> MMVEVRFFGPIKEENFFIKANDLKELRAILQEKEGLKEWLGVCAIALNDHLIDNLNTPLKD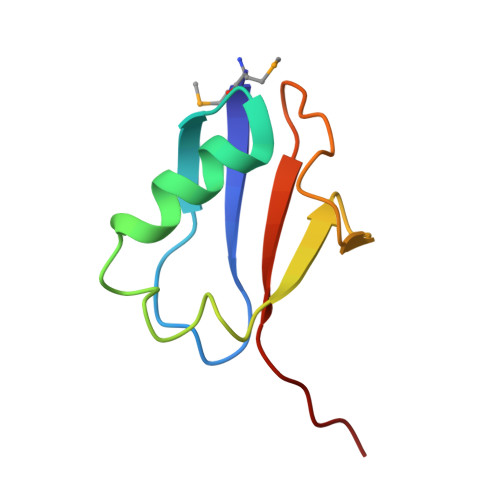GDVISLLPPVCGG>[4x]KETAAAKFERQHMDSSTSAASSSNYCNQMMKSRNLTKDRCKPVNTFVHESLADVQAVCS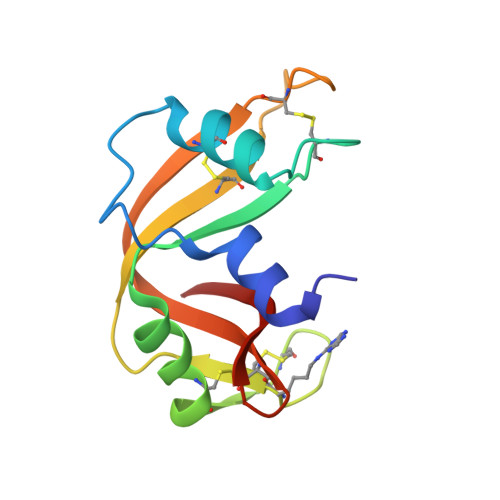QKNVACKNGQTKCYQSYSTMSITACRETGSSKYPNCAYKTTQANKHIIVACEGNPYVPVHFDASV>MSKVVELLKQIQADASVFYVKVHNFHWNVKGMDFHPTHKATQEIYEQFADVFDDVAERVLQLGEMPYVTLADMLKAAKIKEESKTSFCSKEIAQAVLADYEYFLKLFTELSAQADSQGDKVSAAYADDKVGELQKAIWMLKSQLA[12x]

We herein identified the product of the Hc napA gene that we named Cinaedi Atherosclerosis Inflammatory Protein (CAIP), a 200 kDa major antigen of the immune response of Hc-infected individuals with atherosclerosis. DNA-binding proteins from starved cells (Dps) are a group of bacterial miniferritins with a nearly spherical dodecameric structure. With this study we have identified the protein encoded by the napA (IN ITALIC FONT) gene as a novel Hc antigen, which we named Cinaedi Atherosclerosis Inflammatory Protein (CAIP), that possesses a strong immuno-modulatory activity. Collectively, our data suggest that CAIP might be one of the bacterial factors that contribute to the pathogenesis of atherosclerosis associated to Hc infection and that preventing and eradicating the bacterial infection could reduce the incidence of atherosclerosis.

We next crystalized CAIP and characterized its structure. CAIP presents the classical quaternary organization of all the other members of the Dps-like family: a dodecameric shell of over 90 Å in diameter, formed by the twelve subunits arranged with a 32 symmetry. CAIP monomer displays the classical fold of Dps from E. coli, the structural prototype of the family, namely a four-helix bundle, where the second α-helix is connected to the third one through a long stretch of 25 residues; in the middle of the latter a short α-helix is present. Inside the nearly spherical shell formed by the twelve subunits there is an internal cavity of over 40 Å in diameter, where in the other Dps-like proteins iron is stored. As in all the members of the Dps-like family, 12 iron binding sites are present in the putative ferroxidases centres, as detailed in Supplementary Information. The superposition of the equivalent Cα‘s of CAIP to HP-NAP38 indicates that the two proteins are very similar. However, CAIP is very close to HP-NAP produced by H. pylori, as the two proteins have 79% of homology and 58% of identity. CAIP possesses a dodecameric structure similar to that of the other members of the Dps-like family, key factors involved in the protection of prokaryotic cells from oxidative damage, and in particular to that of HP-NAP, a major antigen produced by H. pylori, whose impact on the function of immune cells is well documented. However, the two proteins have an overall identity of 58% and possess a different charge distribution on the surface, which may account for their different properties. In fact, while the exposure of human monocytes to HP-NAP leads to their maturation towards dendritic cells, CAIP-treated monocytes become macrophages and internalize LDL, thereby transforming into foam cells.>SNAMEAFNSWLEGQNLKEQVKNPNIEVGDYSYYSGFYHSKTFEEQAVRYLLGDAPTQEVWESGQFGEVDKLRIGKFCSIASGATFMMAGNQGHRADWISTFPFSKKEFGEGVKDGFQRAGDTIVGNDVWIGSEAMIMPGVHIGDGAIIGARAVITKNVAPYSVVVGNNVVVKKRFDENLIQTLLVIKWWDWPLQHIKNTMEILCSGHIEELEQYF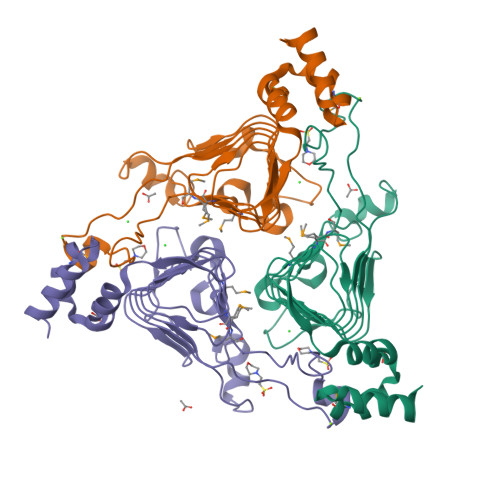IKNVGS[4x]> SNMWVIGKSKAQDAKAIMVNGPQAGWYAPAYTYGIGLHGAGYDVTGNTPFAYPGLVFGHNGVISWGSTAGFGDDVDIFAERLSAEKPGYYLHNGKWVKMLSREETITVKNGQAETFTVWRTVHGNILQTDQTTQTAYAKSRAWDGKELASLLAWTHQMKAKNWQEWTQQAAKQALTINWYYADVNGNIGYVHTGAYPDRQSGHDPRLPVPGTGKWDWKGLLPFEMNPKVYNPQSGYIANWNNSPQKDYPASDLFAFLWGGADRVTEIDRLLEQKPRLTADQAWDVIRQTSRQDLNLRLFLPTLQAATSGLTQSDPRRQLVETLTRWDGINLLNDDGKTWQQPGSAILNVWLTSMLKRTVVAAVPMPFDKWYSASGYETTQDGPTGSLNISVGAKILYEAVQGDKSPIPQAVDLF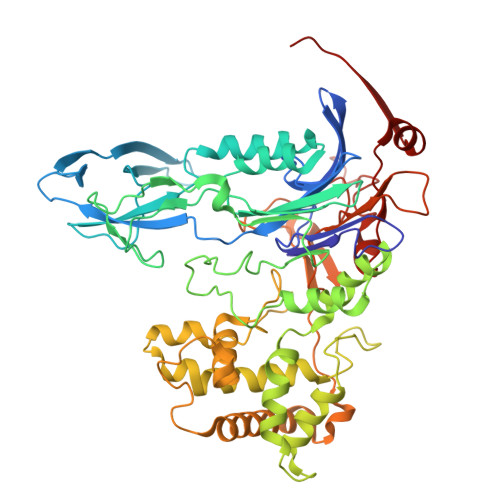AGKPQQEVVLAALEDTWETLSKRYGNNVSNWKTPAMALTFRANNFFGVPQAAAEETRHQAEYQNRGTENDMIVFSPTTSDRPVLAWDVVAPGQSGFIAPDGTVDKHYEDQLKMYENFGRKSLWLTKQDVEAHKESQEVLHVQR> MS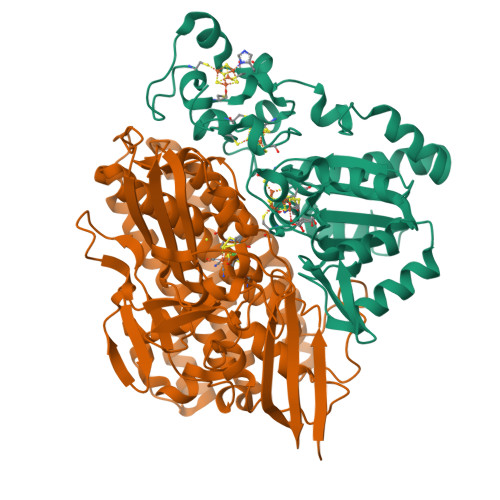LTRRDFVKLCTGTVAGFGISQMFHPAVHEALAGTLTGERPPVFWLQGQGCTGCSVTLLNSVHPSIADVLLKVISLEFHPTVMAWEGEHAIEHMRKVAEKFKGKFFLVIEGSVPVEADGKYCIIGEANHHEISMVDALKEFGPNAAAVLAVGTCAAYGGIPAAEGSETGATAVSKFLGDNGIKTPVVNIPGCPPHPDWIVGTVVLALDAIKKNGLEGGLAEVVKVLDSDGRPTPFFGRNIHENCPYLDKYDEGVMSATFTDKVGCRYDLGCKGPMTMADCFERKWNGGVNWCVQNAVCIGCVEPDFPDGKSPFYQA;> WSHPQFEKGATGRTTIAIDPVTRIEGHLKAEVVVENGKVVDARLSGGMYRGFETILRGRDPRDASQIVQRICGVCPTAHSTASVLALDEAFGAKVPNNGRITRNLIFGANYLQSHILHFYHLSAQDFVQGPDTAPFVPRFPKSDLRLSKELNKAGVDQYIEALEVRRICHEMVALFGGRMPHVQGQVVGGATEIPTKEKLVEYAARFKKVRDFVEQKYVPVVYTIGSKYKDMFKVGQGFKAALCVGAFPLDNSGKKHLFMPGVYAKGKDMPFDPSKIKEYVKYSWFAEETTGLNYKEGKTIPAPDKAGAYSFVKAPRYDGLSLEVGPLARMWVNNPELSPVGKKLLKDLFGISAKKFRDLGEEAAFSLMGRHVARAEETYYMLGAIEGWLKEIKAGEDTVVMPAVPASAEGTGFTEAPRGSLLHYVKVKDSKIDNYQIVSASLWNCNPRDDMGQRGAVEEALIGIPVDDIQNPVNVARLIRAFDPCLGCAVHVLHAESGKVAVIEVK>[4x]MTHPSGEPVYADAVLNGWLTSMGLGVEYVRAEGNTVYYLDDEGREVPVLDHACGFGSLIF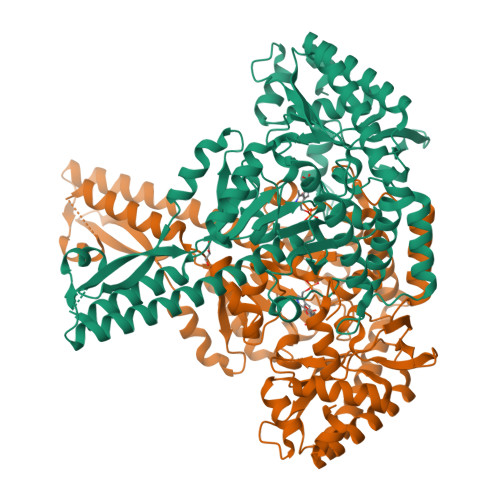GHNHPEIIAHAKAALDAGTVVHAQLSRQPRANQISRILNDIMRRETGRDDRYNAIFANSGAEANEICMKHAELERQERITALFAEIDAELDTAREALTTGTATLDTASLPLVGGGAGDVDGVIADIHRHNDERRAERPLFLTLDGSFHGKLVGSIQLTQNEPWRTPFTALSSPARFLPADEPELIGKIVEDERRSVLTLSLDKDTVRVVERDFPVVAAIFVEPVRGGSGMKTVTPELAEELHRLRDTLGCPLVVDEVQTGIGRTGAFFGSALLGIRGDYYTLAKAIGGGIVKNSVALIRQDRFLPAMEVIHSSTFAKDGLSASIALKVLEMVEADGGRVYQRVRERGQRLEAMLESVRADHSDVVSAVWGTGLMLALELRDQSNATSQAIREKAAHGFLGYVLAGFLLREHHIRVLPAGPRSGFLRFSPSLYITDEEIDRTETALRSLFTALRDQDGDRLVLS> ESQFLKEELVVAVEDVRKQGDLMKSAAGEFADDPCSSVKRGNMVRAARALLSAVTRLLILADMADVYKLLVQLKVVEDGILKLRNAGNEQDLGIQYKALKPEVDKLNIMAAKRQQELKDVGNRDQMAAARGILQKNVPILYTASQACLQHPDV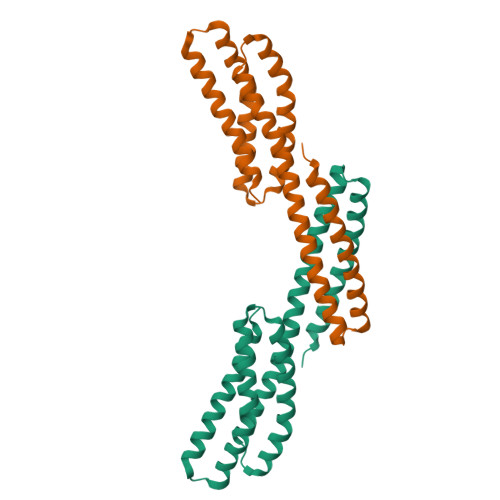AAYKANRDLIYKQLQQAVTGISNAAQAT>[3x]XEWEALEKK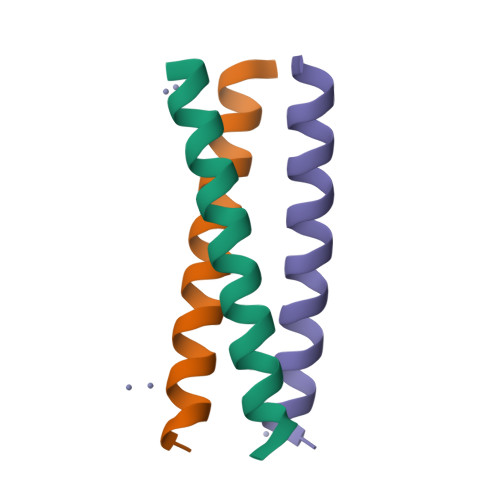LAALESKLQACEKKLEALEHG3-[(1R,2R,3R,5R,6S,7R,9Z,12S,13S,14Z,17S,18S,19R)-2,13,18-tris(2-hydroxy-2-oxoethyl)-3,12,17-tris(3-hydroxy-3-oxopropyl)-3,5,8,8,13,15,18,19-octamethyl-1,2,5,6,7,12,17,22-octahydrocorrin-7-yl]propanoic 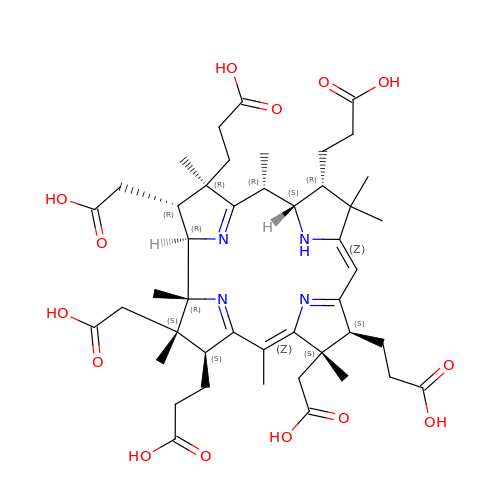acid | C45 H62 N4 O14 | YHLYHOGUCOLFRO-ZWMNGWNLSA-N>[3x]SMKCLFYIAGDVSNYSIVNYELNGQTQNTFFAAHALYNLFKPDKVIALIPDSLVKDNVSDEECYKNLVINRAKELNFAGMEEFMNKVEIRKIPNVGIASAIQCENGAPKKEKNKEGREVLKRLPYNEKRSPIFIFNAIYAIFKDEACDEYLVDLTHGTNVLVSIGMNVGALFNAKFYSAPVMGMPGKDSIVNIVELTDVVQATNDSLMIRSSIENLDERYFKDYSAKLSRLNPTIFEEEEKKVLTRVKGTDVNVVINFLWNIRNGFTVNAVKSMNELKNIINQLEEDLEKLKSFYKNWEEHKNFQGETLLVLSDLDSTLKVKDLLIEGNDLEKLNYLLDLYIKASIYDKALSLARELPVAICLNKVGGGMFDDKNEKYKHCNEIVTSYLRLRYSGLMEFRNTLMHGGLSTDMKPNVDKDGNITPGKIVTKNKIEDFVKRELRNYFDKIVNFLSSA

SisCsx1, as other members of the Csm6/Csx1 family, is composed of an N-terminal CRISPR-Cas-associated Rossmann Fold (CARF) domain connected to an α-helical higher eukaryotes and prokaryotes nucleotide-binding (HEPN) domain by a helix-turn-helix (HTH) domain. The SisCsx1 monomers are curled around the two-fold axis to form a dimer, and three of these dimers oligomerize through their HEPN domains into an equilateral trimer, thus assembling into a hexamer. Each dimer contains a cOA4 binding site at the vertex of the triangular assembly, and a catalytic pocket located 70 Å away inside the triangular oligomer along the two-fold dimer axis. We show that cOA4 binding activates a cooperative sequential catalytic response in a hexameric SisCsx1 complex and that the RNase activity is switched-off by Ring nucleases, which cleave cOA423.

The Cα backbone built in this map was later combined with an iodine derivative of a better diffracting crystal of SisCsx1 in the space group I212121 to determine the structure of the apo SisCsx1 to 2.9 Å. Subsequently the apo SisCsx1 structure was used two determine by molecular replacement two SisCsx1 conformations in complex with cOA4 at 3.1 and 2.7 Å resolution respectively, thus providing the molecular details of the RNase activation by the secondary messenger. To explore these differences, we crystallized the SisCsx1-cOA4 complex by soaking the compound in crystals of the apo SisCsx1 at 25 °C, and we also co-crystallized the complex after heating up the mixture of cOA4 with the isolated SisCsx1 to monitor possible conformational changes that could elicit the RNase activity by the presence of cOA4. We synthesized cOA4 using purified Type III-B SisCmr−α complex, and observed that the binding of cOA4 at room temperature, barely activates SisCsx1, while heating the reaction mixture triggered full RNase activity. The phosphate inversion in cOA4 is stabilized in both cases by hydrogen bonds of the phosphate groups of A1 and A3 with N158 and N158′ through a water molecule. A rotamer change of H155 in both monomers allows the polar interaction of the imidazole group with the A2 and A4 bases in each monomer, thus positioning the cyclic compound into the cruciform pocket. In addition, A2 and A4 phosphates are stabilized by the side chains of Y14 and Y14′. Finally, the anti conformation of A2 and A4 is stabilized by interactions of the base with the main chain of S15, S15′, F29′, and V180′ and the OH of Y19′, while the syn configurations observed for A1 and A3 are stabilized by polar interactions with the main chain of D10, D10′, S51, S51′, and S98 and hydrophobic contacts with M181 side chain in both monomers.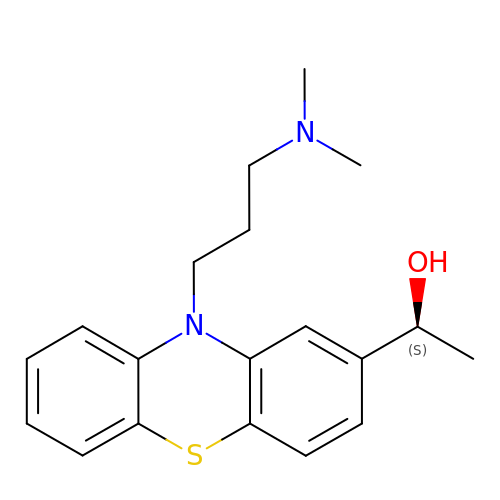(1~{S})-1-[10-[3-(dimethylamino)propyl]phenothiazin-2-yl]ethanol | C19 H24 N2 O S | ZIJWCRNUEBJMSQ-AWEZNQCLSA-N> MIVPVLSRQALRHASVARVALPSLTRWYASYPPHTVVKMPALSPTMTSGGIGAWQKKPGDKIEPGEVLVEIETDKAQMDFEFQEEGVLAKILKDSGEKDVAVGNPIAILVEEGTDVNAFKDFTLKDAGGETSPAVPKDEPKNESTASAPTPAPTPAPEPENTSFTGRFQTALEREPNALPAAKRLAREKGIDLRNVKGSGPGGKITEEDVKKALASAPAAGAAAAAYTDVPISGMRKTIAARLKESVTENPHFFVSTNLSVSKLLKLRQA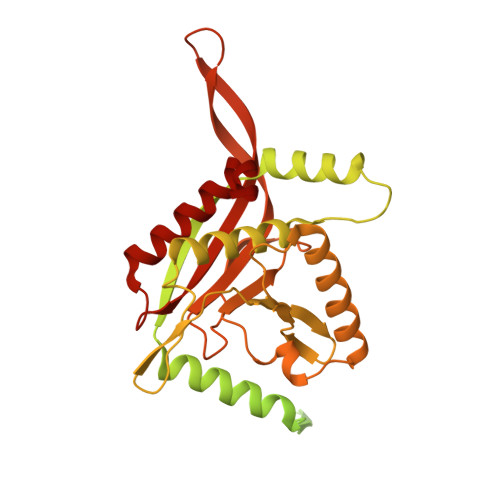LNSSADGRYKLSVNDFLIKAMGIASKRVPTVNSSWRDGVIRQFETVDVSVAVATPNGLITPIVKGVEGKGLESISAAVKELAKKARDGKLKPEEYQGGSISISNMGMNPAVQSFTAIINPPQAAILAVGAPQKVAVPVENEDGTTGVSWDEQIIVTASFDHKVVDGAVGAEWIRELKKVIENPLELLL>GPFRGRIELIIGPMFAGKTTELMRRVKREIHARRSCFVIKYSKDTRYDEHNVASHDQLMLRAQAAVSQLTEVRDTWKRFDVLAI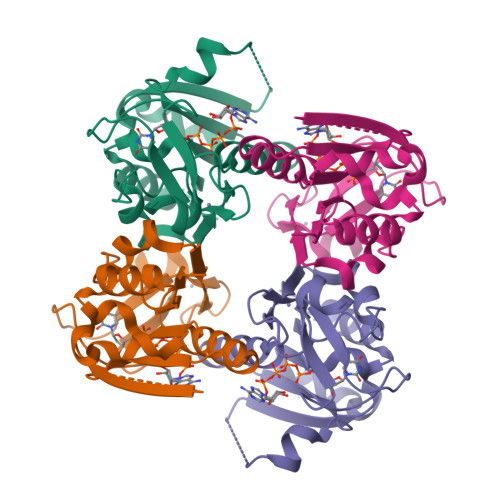DEGQFFSDLVDFCNTAADAGKVVMVSALDGDYRRKPFGQICELVPYCEAVDKLTAVCMMCHEQPACFTRRTVNVEQQELIGGADMYIATCRECYSKQQLP[2x]>SLSHKAWQNAHAMYENDACAKALGIDIISMDEGFAVVTMTVTAQMLNGHQSCHGGQLFSLADTAFAYACNSQGLAAVASACTIDFLRPGFAGDTLTATAQVRHQGKQTGVYDIEIVNQQQKTVALFRGKSHRIGGTITGEA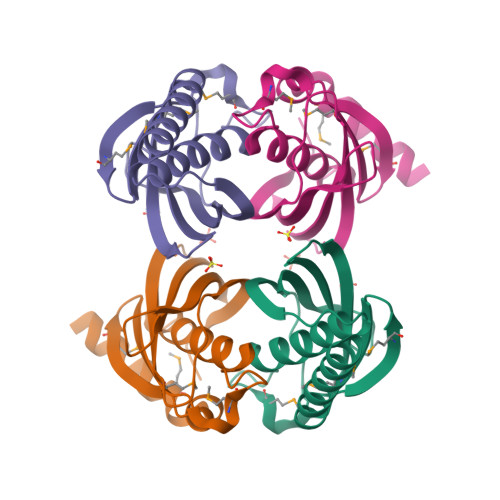EGGSHHHHHH[2x]> FNLDTEELTAFRVDSAGFGDSVVQYANSWVVVGAPQKITAANQTGGLYQCGYSTGACEPIGLQVPPEAVNMSLGLSLASTTSPS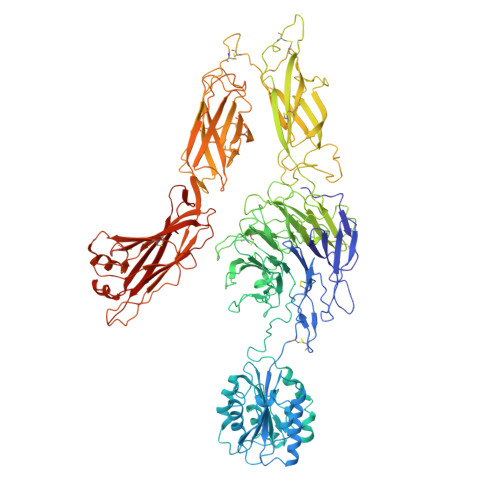QLLACGPTVHHECGRNMYLTGLCFLLGPTQLTQRLPVSRQECPRQEQDIVFLIDGSGSISSRNFATMMNFVRAVISQFQRPSTQFSLMQFSNKFQTHFTFEEFRRSSNPLSLLASVHQLQGFTYTATAIQNVVHRLFHASYGARRDAAKILIVITDGKKEGDSLDYKDVIPMADAAGIIRYAIGVGLAFQNRNSWKELNDIASKPSQEHIFKVEDFDALKDIQNQLKEKIFAIEGTETTSSSSFELEMAQEGFSAVFTPDGPVLGAVGSFTWSGGAFLYPPNMSPTFINMSQENVDMRDSYLGYSTELALWKGVQSLVLGAPRYQHTGKAVIFTQVSRQWRMKAEVTGTQIGSYFGASLCSVDVDSDGSTDLVLIGAPHYYEQTRGGQVSVCPLPRGWRRWWCDAVLYGEQGHPWGRFGAALTVLGDVNGDKLTDVVIGAPGEEENRGAVYLFHGVLGPSISPSHSQRIAGSQLSSRLQYFGQALSGGQDLTQDGLVDLAVGARGQVLLLRTRPVLWVGVSMQFIPAEIPRSAFECREQVVSEQTLVQSNICLYIDKRSKNLLGSRDLQSSVTLDLALDPGRLSPRATFQETKNRSLSRVRVLGLKAHCENFNLLLPSCVEDSVTPITLRLNFTLVGKPLLAFRNLRPMLAADAQRYFTASLPFEKNCGADHICQDNLGISFSFPGLKSLLVGSNLELNAEVMVWNDGEDSYGTTITFSHPAGLSYRYVAEGQKQGQLRSLHLTCDSAPVGSQGTWSTSCRINHLIFRGGAQITFLATFDVSPKAVLGDRLLLTANVSSENNTPRTSKTTFQLELPVKYAVYTVVSSHEQFTKYLNFSESEEKESHVAMHRYQVNNLGQRDLPVSINFWVPVELNQEAVWMDVEVSHPQNPSLRCSSEKIAPPASDFLAHIQKNPVLDCSIAGCLRFRCDVPSFSVQEELDFTLKGNLSFGWVRQILQKKVSVVSVAEITFDTSVYSQLPGQEAFMRAQTTTVLEKYKVHGCGGLENLYFQ>MSISWTRNFFERFCVEEYNIDTIKQSSFLSADLLPSLGARINQSTKLRKHIISPFNPRYRAWEMWLVLLVIYSAWICPFQFAFITYKKDAIFIIDNIVNGFFAIDIILTFFVAYLDSHSYLLVDSPKKIAIRYLSTWFAFDVCSTAPFQPLSLLFNYNGSELGFRILSMLRLWRLRRVSSLFARLEKDIRFNYFWIRCTKLISVTLFAIHCAGCFNYLIADRYPNPRKTWIGAVYPNFKEASLWNRYVTALYWSITTLTTTGYGDFHAENPREMLFDIFFMMFNLGLTAYLIGNMTNLVVHWTSRTRTFRDSVRAASEFASRNQLPHDIQDQMLSHICLKFKTEGLKQQETLNNLPKAIRSSIANYLFFPIVHNIYLFQGVSRNFLFQLVSDIDAEYFPPKEDIILQNEAPTDLYILVSGAVDFTVYVDGHDQFQGKAVIGETFGEVGVLYYRPQPFTVRTTELSQILRISRTSLMSAMHAHADDGRVIMNNLFMKLRGQQSIAIDDSNTSGHENRDFKSMGWEEWRDSRKDGYGLDVTNPTSDTALMDAIHKEDTEMVKKILKEQKIERAKVERSSSETAGRSYANDSSKKDPYCSSSNQIIKPCKREEKRVTIHMMSESKNGKLILLPSSIEELLRLASEKFGGCNFTKITNADNAEIDDLDVIWDGDHLYFSSN[4x]

KAT1 is a voltage-dependent potassium channel from Arabidopsis thaliana that is mainly expressed in guard cells. KAT1 allows the influx of K+, leading to the swelling and opening of the stoma, and therefore plays a key role in regulating the aperture of stomatal pores on the surface of plant leaves. Comparing with conventional depolarized K+ channels, KAT1 has a uniquely reversed voltage dependence: depolarization causes closing, and hyperpolarization causes opening. KAT1 thus falls into a rare class of hyperpolarization-activated channels, which include hyperpolarization-activated, cyclic nucleotide-gated (HCN) channels in animals, and KAT and AKT channels in plants.

A three-dimensional EM map was reconstructed to an overall resolution of 3.2 Å. Cryo-EM structure shows that KAT1 assembles as a tetramer channel with a 4-fold symmetry. Each subunit contains a voltage sensor domain (VSD, helices S1–S4) and a pore-forming region (helices S5–S6) inside the membrane bilayer. Each VSD of KAT1 is contiguous with the pore domain from the same subunit, and connected to the pore domain through a short, non-helical turn (named S4–S5 linker). The pore domain displays a closed inner gate, with its narrowest constriction formed by the hydrophobic side chains of Ile292. The conductive conformation of the selectivity filter and the closed gate correspond to the expected closed state of KAT1 at 0 mV. The structure of KAT1 shows that the middle of the S4 helix adopts a 310 conformation, whereas the upper and lower parts are α-helices. We also found that the positive charges of the depolarization-gated channels Kv1.2-2.1 and Eag1 are mostly distributed in the upper part of the S4 helix, while the positive charges of KAT1 are mostly distributed in the lower part of the S4 helix. In KAT1, the short, non-helical S4–S5 linker contacts the C-linker of a neighboring subunit through electrostatic and hydrophobic interactions. We found that mutations of residues located in the S4–S5 linker, Ile189Ala and Arg310Ala, disrupt channel opening, while the Ile189Val mutation leads to a decreased current from KAT1 upon hyperpolarization.> SAAGAAQFLDQLLPKTAGVSSPEQVLIEEIKKRHLATASGGSGGSGGSSDCFEITGKAYNIDPLILKAIAWNESKNKNGIKSKINKNGTYDIGIMQINSSHLDLLSKFNISEDDLLNDACINISVAGYILASNIKSRGNTWDAVGAYNAGYFNTPNAV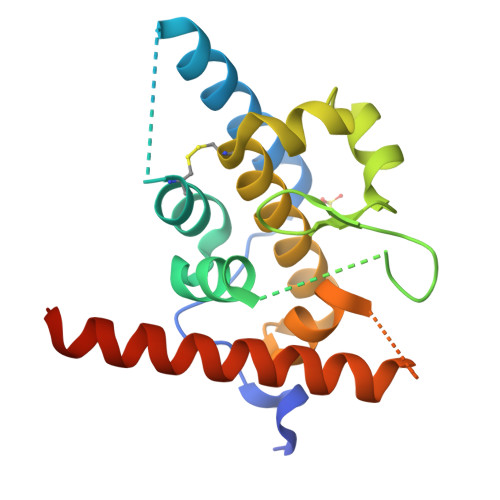ELRRQYAMKIYKTYTKLKNNEQIIDHHHHHH>MSLAHTAAEYMLSDALLPDRRGPRLKGLRLELPLDRIVKFVAVGSPLLLMSLAFAQEFSSGSPISCFSPSNFSIRQAAYVDSSCWDSLLHHKQDGPGQDKMKSLWPHKALPYSLLALALLMYLPVLLWQYAAVPALSSDLLFIISELDKSYNRSIRLVQHMLKIRQKSSDPYVFWNELEKARKERYFEFPLLERYLACKQRSHSLVATYLLRNSLLLIFTSATYLYLGHFHLDVFFQEEFSCSIKTGLLSDETHVPNLITCRLTSLSIFQIVSLSSVAIYTILVPVIIYNLTRLCRWDKRLLSVYEMLPAFDLLSRKMLGCPINDLNVILLFLRANISELISFSWLSVLCVLKDTTTQKHNIDTVVDFMTLLAGLEPSKPK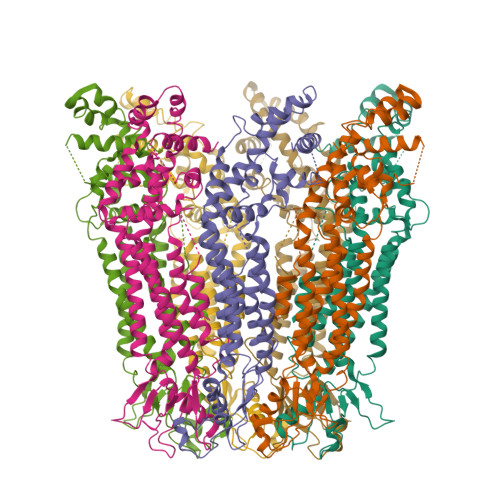HLTNSACDEHP[7x]> VSSCSEDWVGYQRKCYFISTVKRSWTSAQNACSEHGATLAVIDSEKDMNFLKRYAGREEHWVGLKKEPGHPWKWSNGKEFNNWFNVTGSDKCVFLKNTEVSSMECEKNLY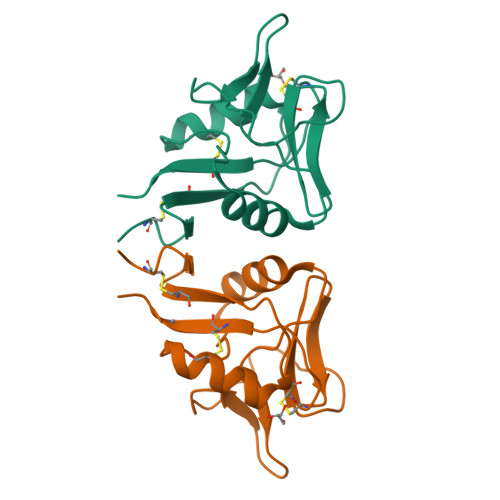WICNKPYK> GAASPKQ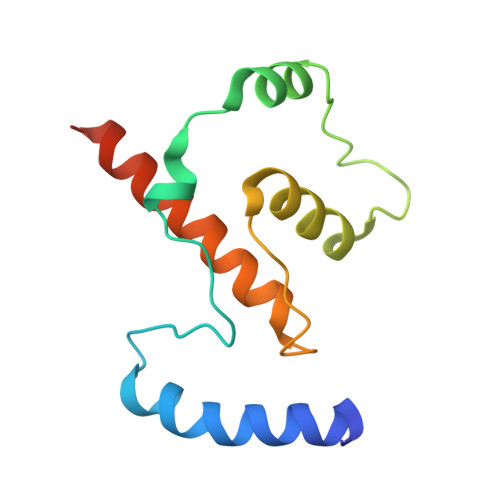IQMWINNVAEIRKTKQPHSVSYTKPMPEIDELMQEWPQEIEEILQHLKIPSEELDFNLSDFCKLACAILDIPVHDQPNESNVIESLHVLFTLYSEFKSNQHFQQNKNDG> MYEGRWKMVNQIKQDVQNDIELILRQMNERIHAMKKKKYNELKGKIKQKCIDLLIDYAKQKIGKKNKIKKEGNNIRHNKQKKLKNIQKKIFKIISTRMLQTTLSAFRPRGSNVTGKVALATLGALTGYGAFYHYNQYLNLSARWQQIQENIAKDQPF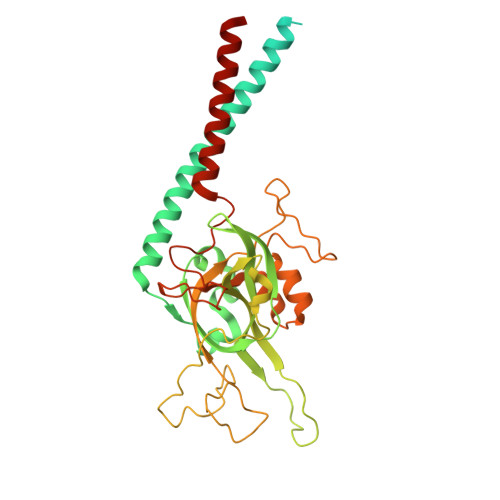DVDGFDAKVYPWVRENNVNDWEYKLVKMRGYFKDQRFFVRRKRDGKEGFLVFAPFVTAVERVNHRLKQKDLLPVEYSVFVNLGWVPVENKKDVELGGEVCPPMDAPTDSTLFVNDTFTGFNPDPANPEDTEQVTLTEITGIVRRGEQQDILARRRNWNKEGIYNWVDLDYMGKIFRLFNLDAINTAYIERVVPSFEEGEEGLYPIPATKDTFERPLNTPERHSTFFNFYAATSALSFISMLLLRR> MKVSYIFSFFLLFFVYKNTNTVVCDNGYGDLAATSALTTVIKDPISLTIKDIYEHGVKNPFTKII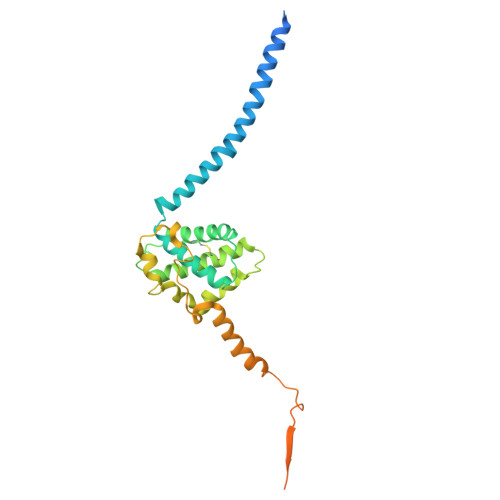HKLKKFIRYRKVLRWSRMWWVLLVREIVGDNTIEKKTEKALREIWDQCTIAVYNNTLNAVESKPLLFLHGILNECRNNFATKLRQDPSLIVAKIDQIIKSQIYRFWVSEPYLKIGRSHTLYTHITPDAVPQLPKECTLKHLSSYMEEKLKSMESKKNIESGKYEFDVDSSETDSTKDDGKPDDDDDDDDNFDDDDNFDDDTVEEEDASGDLFKNEKKDENKE>[2x]MHHHHHHGMNAIKLYPLKKLEIILEGAHKEFATDLLDRAGVKGY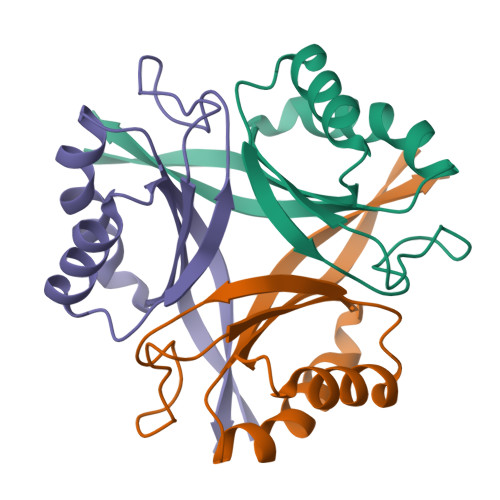TIVGNLSGKGSHGMYEGHLMFNEDDALIMIIAAVPEELVGPLLEGFQPFFEAHSGVVFVHDIQVGRPIKFRN> LGAAVAFPVDDDDKIVGGYTCGANTVPYQVSLNSGYHFCGGSLINSQWVVSAAHCYKSGIQVRLG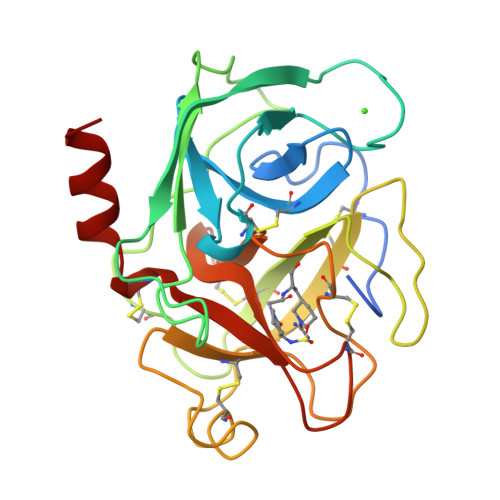EDNINVVEGNEQFISASKSIVHPSYNSNTLNNDIMLIKLKSAASLNSRVASISLPTSCASAGTQCLISGWGNTKSSGTSYPDVLKCLKAPILSDSSCKSAYPGQITSNMFCAGYLEGGKDSCQGDSGGPVVCSGKLQGIVSWGSGCAQKNKPGVYTKVCNYVSWIKQTIASN> MVKVLFFAQVRELVGTDATEVAADFPTVEALRQHMAAQSDRWALALED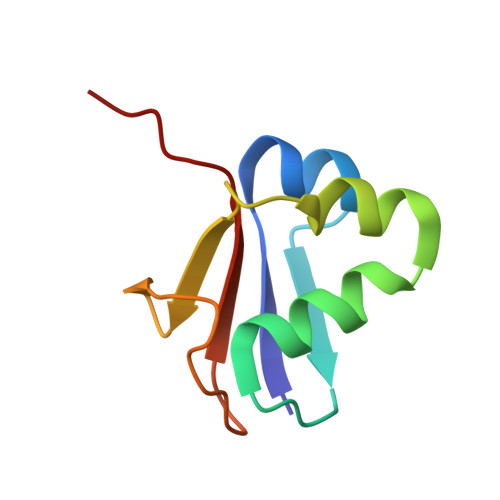GKLLAAVNQTLVSFDHPLTDGDEVAFFPPVTGG>[2x]MKEVVIASAVRTAIGSYGKSLKDVPAVDLGATAIKEAVKKAGIKPEDVNEVILGNVLQAGLGQNPARQASFKAGLPVEIPAMTINKVCGSGLRTVSLAAQIIKAGDADVIIAGGMENMSRAPYLANNARWGYRMGNAKFVDEMITDGLWDAFNDYHMGITAENIAERWNISREEQDEFALASQKKAEEAIKSGQFKDEIVPVVIKGRKGETVVDTDEHPRFGSTIEGLAKLKPAFKKDGTVTAGNASGLNDCAAVLVIMSAEKAKELGVKPLAKIVSYGSAGVDPAIMGYGPFYATKAAIEKAGWTVDELDLIESNEAFAAQSLAVAKDLKFDMNKVNVNGGAIALGHPIGASGARILVTLVHAMQKRDAKKGLATLCIGGGQGTAILLEKCLEHHHHHH

Here, we present the crystal structure of C. acetobutylicum thiolase (CaTHL), a type II biosynthetic thiolase that catalyses the first step of n-butanol biosynthesis and condenses two acetyl-CoAs to acetoacetyl-CoA. We reveal that CaTHL, unlike other type II biosynthetic thiolases from aerobic bacteria, is regulated via modulation of a redox-switch, indicating that n-butanol production and the relevant metabolic fluxes in Clostridium are tightly regulated by thiolase. CaTHL consists of three domains: an N-terminal α/β domain (N-domain, residues 1–119 and 249–269), a loop domain (L-domain, residues 120–248), and a C-terminal α/β domain (C-domain, residues 270–392). The N- and C-domains form a typical five-layered fold (α–β–α–β–α) observed in other thiolase superfamily of proteins including peroxisomal degradative thiolase from Saccharomyces cerevisiae, β-ketoacyl synthase II from E. coli, and the biosynthetic thiolase from Zoogloea ramigera (ZrTHL)14151617181920.

The 1.77 Å crystal structure of CaTHL was determined to understand the structural basis for its catalytic and regulatory mechanisms. The asymmetric unit contains two CaTHL molecules, and the tetrameric structure of the protein could easily be generated by applying crystallographic P21212 symmetry. Interestingly, under oxidized conditions, a disulfide bond was formed between two catalytic cysteine residues (Cys88 and Cys378) in CaTHL. Such disulfide bond formation has not been reported in other type II biosynthetic thiolases. The disulfide bond formation was followed by a large conformational change in the catalytic cysteine loop (CIGGGQG, residues 378–384). The Cys378 residue rotates 180° towards the Cys88 residue via the rotation of the peptide bond between Leu377 and Cys378, which in turn induces a movement of the catalytic cysteine loop away from the active site. The consequence of this conformational change in the catalytic cysteine loop is that the region between β11 and α10 (SAGVDPAIMGYGP, residues 280–292) becomes disordered due to the steric clash. Hereafter, this disordered region will be referred to as the flexible region. In summary, the oxidized CaTHL becomes inactive due to the oxidation of both catalytic cysteine residues accompanied by large conformational changes in the catalytic cysteine loop and the flexible region. Interestingly, in the oxidized form of CaTHL, the conformational change between the ‘catalytic cysteine loop' and the ‘RDR' forms a hole that enables the cellular reductants to access to the disulfide bond.> NTPIPRRHT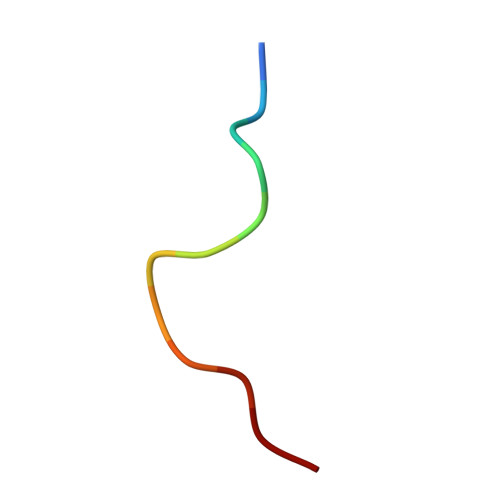RSA>GSEQLGELMEPALGYVVKVPVSSFENKKVDISDIEVITNGNLDDVPYKANSSKYNYPDIKTKDSSLQYVRSGYVIDGEHSGSNEKGYVYYKGNSP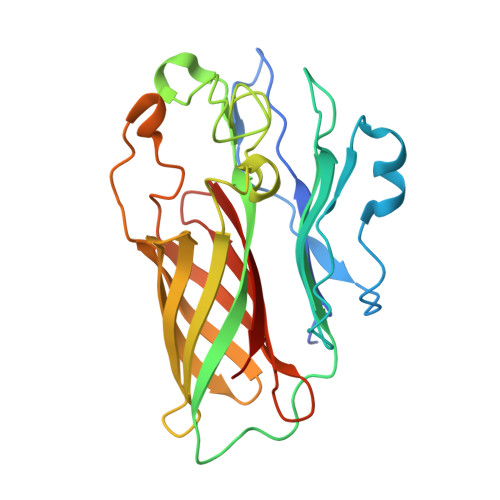AKELPVNQLLTYTGSWDFTSNANLNNEEGRPNYLNDDYYTKFIGKRVGLVSGDAKPAKHKYTSQFEVDFATKKMTGKLSDKEKTIYTVNADIRGNRFTGAATASDKNKGKGESYNFFSADSQSLEGGFYGPKAEEMAGKFVANDKSLFAVFSAKHNGSNV[2x]2-[[(2~{S})-3-naphthalen-1-yloxy-2-oxidanyl-propyl]amino]propane-1,3-diol | C16 H21 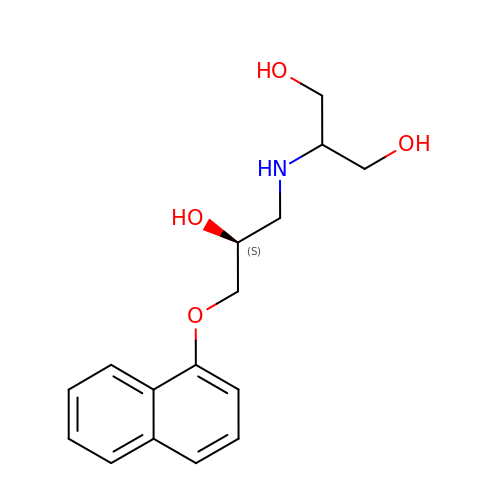N O4 | KRBDCALBFRZJTM-AWEZNQCLSA-N2-[[6-(5-azanyl-1~{H}-pyrazol-3-yl)indol-1-yl]methyl]benzenecarbonitrile | C19 H15 N5 | 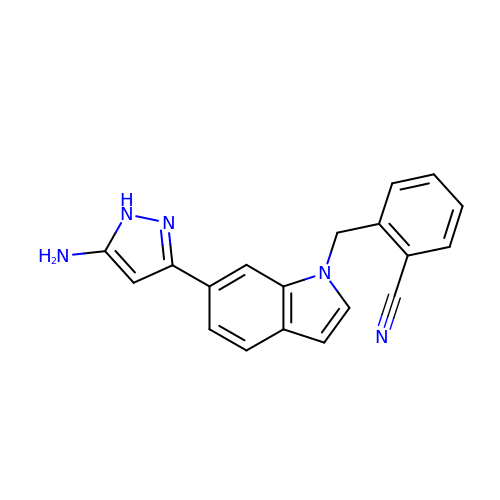BIAUTOGYZPQBHF-UHFFFAOYSA-N>MHHHHHHHHENLYFQGPTEQTHNVVHEANGVKLRETPKEFFERQPNKGHIHDVNQYKQMYEQSIKDPQGFFGPLAKELLSWDHDFHTVKSGTLKNGDAAWFLGGELNASYNCVDRHAFANPDKPALICEADDEKDSHILTYGDLLREVSKVAGVLQSWGIKKGDTVAVYLPMNAQAIIAMLAIARLGAAHSVIFAGFSAGSIKDRVNDASCKALITCDEGKRGGRTTNIKKLCDEALVDCPTVEKVLVYKRTNNPEIHLTEGRDYYWDVETAKFPGYLPPVSVNSEDPLFLLYTSGSTGTPKGVVHSTAGYLLGAALSTKYIFDIHPEDILFTAGDVGWITGHTYALYGPLLLGVPTIIFEGTPAYPDYGRFWQIVEKHKATHFYVAPTALRLLRKAGEQEIAKYDLSSLRTLGSVGEPISPDIWEWYNEFVGKNQ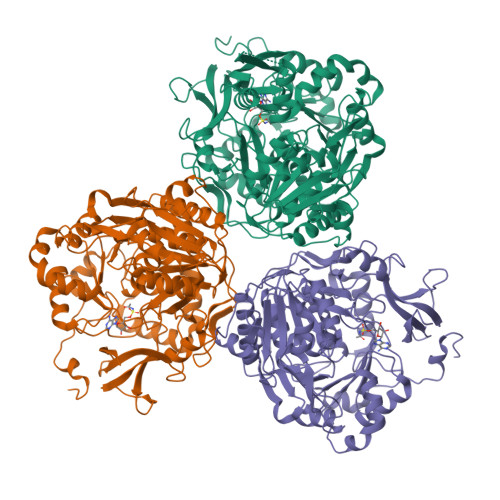CHISDTYWQTESGSHLIAPLAGVVPNKPGSASYPFFGIDAALIDPVTGVEIEGNDAEGVLAIKDHWPSMARTVYKNHTKYMDTYMNPYPGYYFTGDGAARDHDGYYWIRGRVDDVVNVSGHRLSTAEIEAALIEDKKVSEAAVVGIHDDITGQAVIAYVALKEGNSDEDSEGLRKELVLQVRKTIGPFAAPKSVIIVQDLPKTRSGKIMRRILRKVSSNEADQLGDISTLSNPQSVEGIISAFGAQFGKK[3x]> GSDYIIKEKTVLLQKKDSEGFGFVLRGAKAQ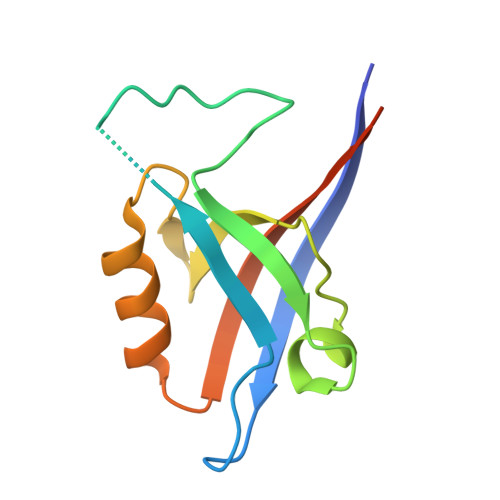TPIEEFTPTPAFPALQYLESVDEGGVAWRAGLRMGDFLIEVNGQNVVKVGHRQVVNMIRQGGNTLMVKVVMVTRHPDMDEAVHK Purine nucleoside phosphorylase (PNP, purine nucleoside orthophosphate ribosyl transferase, EC 2.4.2.1) has a crucial role in the purine salvage pathway. It catalyses the reversible phosphorolytic cleavage of the glycosidic bond of purine (2′-deoxy) nucleosides, generating the corresponding free base and (2′-deoxy) ribose 1-phosphate. E. coli PNP is an excellent molecular machine conducting efficient catalysis of purine nucleosides glycosidic bond cleavage. It is a homohexamer, built as a trimer of dimers, with all its subunits having the active site in the open conformation in the apo enzyme form. Monomers in each dimer mutually donate two amino acids (His4 and Arg43) to complete their active sites.

In the case of orthorhombic structures of the wild-type enzyme with two formycin molecules (WT-6(P/S)-2FA) and of the double mutant complexes with two and four formycin molecules per hexamer bound, (DM-6(P/S)-2FA and DM-6(P/S)-4FA, respectively) all six monomers are crystallographically independent, whereas in the case of hexagonal structures of the wild-type and the mutant with six formycin molecules bound by each hexamer (WT-6(P/S)-6FA and DM-6(P/S)-6FA) two halves of the hexamer are related by the crystallographic two-fold axis. In the orthorhombic structures, dimers A-D and F-C are closed-open dimers and B-E form an open-open dimer, while in the hexagonal forms A-D is the closed-open dimer and B-B’ is the open-open dimer formed by crystallographic two-fold symmetry. In the structure of WT-6(P/S)-2FA, the FA molecules are found only in the closed active sites A and F with final occupancies of 0.7. All of the active sites in the open conformation in this complex are occupied only by water molecules. This is the first time that the presence of nucleoside type substrate only in the active sites in closed conformations was shown. In the case of WT, at low nucleoside concentrations, the nucleoside is bound mostly in sites adopting a closed conformation, which facilitates protonation, hence also catalysis.

>ATPHINAEMGDFADVVLMPGDPLRAKYIAETFLEDAREVNNVRGMLGFTGTYKGRKISVMGHGMGIPSCSIYTKELITDFGVKKIIRVGSCGAVLPHVKLRDVVIGMGACTDSKVNRIRFKDHDFAAIADFDMVRNAVDAAKALGIDARVGNLFSADLFYSPDGEMFDVMEKYGILGVEMEAAGIYGVAAEFGAKALTICTVSDHIRTHEQTTAAERQTTFNDMIKIALESVLLGDK[6x]> AEETCFDKYTGNTYRVGDTYERPKDSMIWDCTCIGAG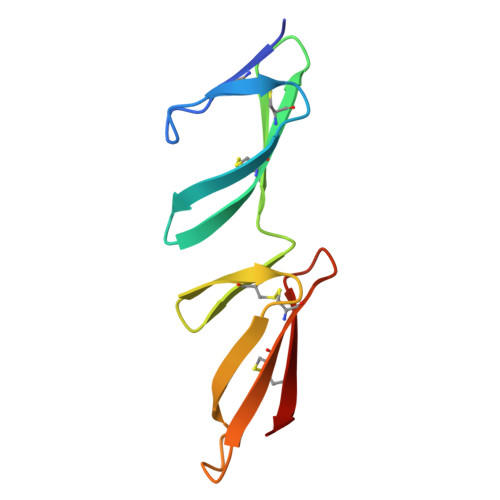RGRISCTIANRCHEGGQSYKIGDTWRRPHETGGYMLECVCLGNGKGEWTCKPI> SLDTEKDCIKAVAAKD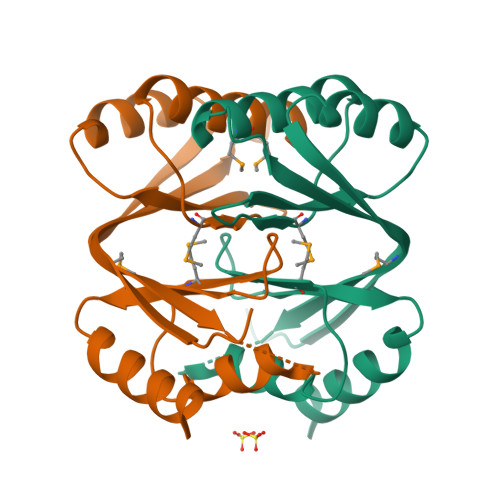GITVIKVKSSNKLLSWHFMRKLFEIFEFYQEPVDMVATSEVGVSLTIDNDKNLPDIVRALSDIGDVTVDKDMVIICIVGDMEWDNVGFEARIINALKGVPVRMISYGGSNYNVSVLVKAEDKKKALIALSNKLFNSRATKA>GSHMASKGNIEVLNLVTGPDSITTIELYLNTRMGQNDESKDNYGYSEKVTVANSSDQDKPTSGEIPTYSTARINLPMLNEDLTCNTLTMWEAVSVKTEV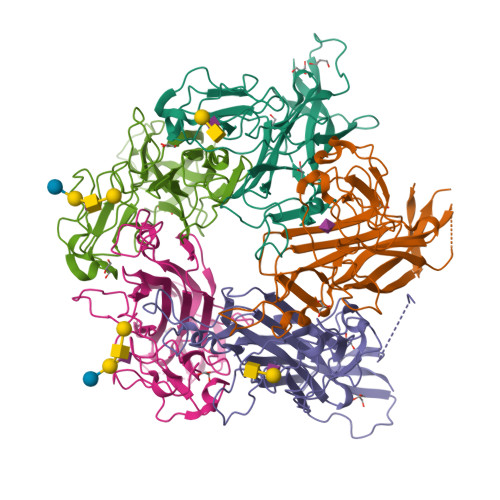VGVSSLVNVHMATKRMYDDKGIGFPVEGMNFHMFAVGGEPLELQFLTGNYRTDYSANDKLVVPPIKHQSTQGLNPHYKQKLTKDGAFPVECWCPDPSKNENTRYYGSYTGGQSTPPVLQFTNTVTTVLLDENGVGPLCKGDGLYVSCCDIVGFLVGKDGDMQYRGLPRYFNILLRKRTVRN[5x]5-bromo-3-methyl-1H-indole-2-carboxylic 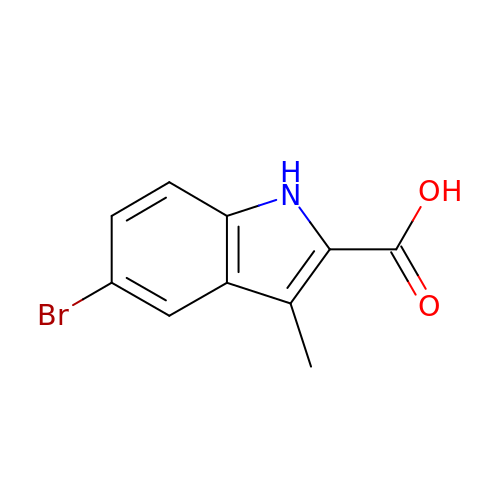acid | C10 H8 Br N O2 | YUMRTSLYUVLHQK-UHFFFAOYSA-N> MSLYEHAALPLASSPSILGPISGGRNRGNIQLQSIPIEFQAVVFAGFGNSLYPLTGSDALPKALLPIGNKPMLHYPLYWLEAAGFTSAILICMEEAEAHINAWLRSGYEGHMRIHVEAPTILDDSKSSADALRAVSHLIKNDFVCLSCDSIVGLPPYTVLDKFRLDNPSALAVYSPVLKYEHITSQSKEIDAKQLIGIEEKTSRLLYAKSSADVGSDFTFRMSLLWKHPRVTLNTNLSDAHIFVFKHWVIDLIREKESISSIRGDLIPYLVKCQYQKSFTVRENIQRFLSSPNNIDNYDGGLSSQEIKINALIAKDGIICSRANNLPNYFELNKCIAKLTPEQRLVDVTVSERALVGADCMVNEGTTIKDNSNIKKSIIGKNCVIGKGVVVSNSILMDNIVVEDGVRLESCIVASGAQIGAKSKLRECE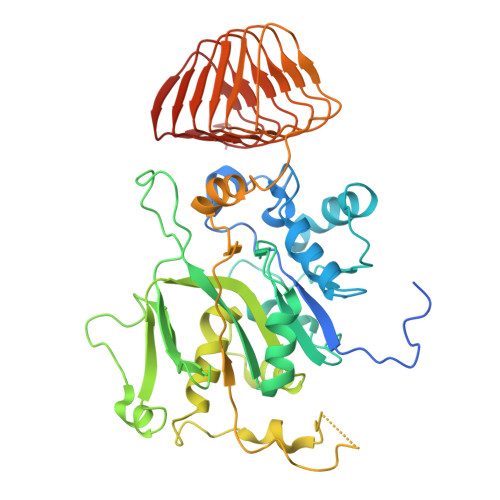IGVDHRVEAGRIARGERLVDMEKIETDMD> MRAAPTRLAPSTVASLGRSHCGSQAYHLDAAGAAGWRR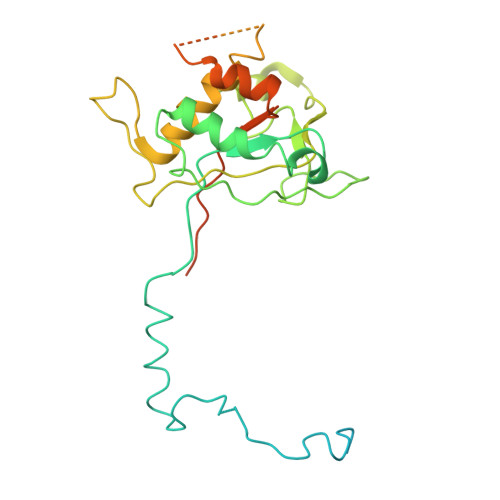RRRLTGVSMTTTHTVAPAVSALPFSLSTARRTYYWPYPENLVPEGATTSPFQSSPVPSVRERIIREYALGPLFGSRTPCCVLGFAGTARDVAACKRDVRRWVARALGKSEADVELGALVQAKEMLLHRSGTDESPRLGDGPGSRPDAEQRRVTRYARLPVQARTLLEVYLPGEEHGEVDAAADADATILAHGYFLQEQLHRHMTTTASSGSDPTGRRDSEDCQPEEPARKMQSHCQGCSEPNDEADVKSSVAALHDVCGVIYCEVPVLDESDFAFDQLCGKEVDDETTERVTDRWTRRAMQQQPQL>MLQNSFKLAQSLRNGFYRNAWRAFSSHGPRQPLVSPERRLEKAHPTFTERSQLKYARRLVVKLGSAVITREDNHGLALGRLASIVEQVAECHLEGREVMMVTSGAVAFGKQKLAQELLMSLSMRETLNPKDSKEFDGATLEPRAAAAVGQSGLMSLYDAMFAQYGVKIAQVLVTKPDFYNEETRNNLFCTLSELISLNIVPIINTNDAVSPPMFIRDDEPAGGARRGIPIKDNDSLSAMLAAEVQADLLILMSDVDGIYNKPPWEDGAKLMHTYTSDDSNSIEFGKKSKVGTGGMDSKVKAATWALDRGVSVVICNGMQEKAIKTIIGGRKVGTFFTEATESANAVPVEVMAENARTGSRQMQALTPAQRASAVNTLADLLVSREKFILDANAKDLAEAQKSGLAKPLLSRLSLNPAKLKNLSVGLKQIAEDSHKNVGRVLRRTRLADQLELKQVTVPIGVLLVIFESRPDSLPQVAALAMASANGLLLKGGKEAAHSNKALMELVKEALATVGAEHAVSLVSTREEISDLLSMENHIDLIIPRGSSDLVRSIQQQSLHIPVLGHAEGVCHVYIDRDADLEKALRIARDAKCDYPAACNAMETLLIHEDLMSGAIFGDVCNMLKREGVKIYAGPRLNQQLTFGPPAAKSLKHEYGALECCIEVVPSLDEAINHIHTYGSSHTDVIVTENDAAARQFLGSVDSACVFHNASSRFADGFRFGLGAEVGISTARIHARGPVGVEGLLTTKW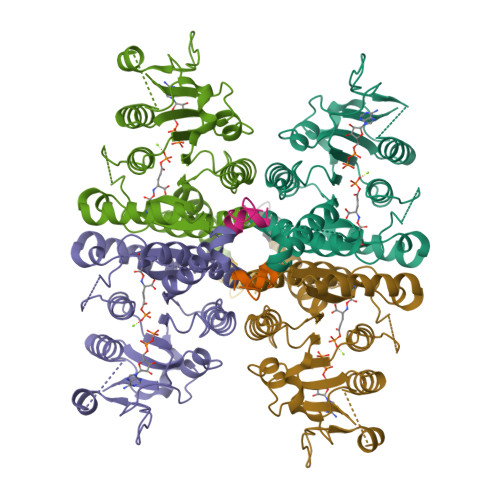ILEGQDHAAADFAEGGGRTWLHETLPLD[8x]>SADVAGAVIDGAGLGFDVLKTVLEALGNVKRKIAVGIDNESGRTWTAMNTYFRSGTSDIVLPHKVAHGKALLYNGQKNRGPVATGVVGVIAYSMSDGNTLAVLFSVPYDYNWYSNWWNVRVYKGQKRANQRMYEELYYHRSPFRGDNGWHSRSLGYGLKSRGFMNSSGHAILEIHVTKA[2x]

The multigene family of actinoporins are a group of cnidarian pore-forming toxins produced by sea anemones well known for their widespread polymorphism. Strongly influenced by negative selection, actinoporins have conserved important functional sites to ensure the preservation of their mechanism of pore formation, a complex process involving many different steps. The steps leading to pore formation comprise (1) the binding of the toxins to the cell membrane, (2) toxin diffusion across the membrane plane, (3) protein oligomerization, and (4) translocation of the N-terminal α-helices through the lipid bilayer.

The structure is composed of a β-sandwich core flanked by an N-terminal and a C-terminal α-helix. Relevant functional areas such as the lipid-binding region (contoured by a hydrophobic loop and the C-terminal α-helix) and the pore-forming N-terminal α-helix were conserved. When considering only the differences among fragaceatoxins, it is observed that FraE shared a high identity (98%) with FraC, explaining their similar activity above. The most stable isoforms were FraA and FraB as judged by their higher TM values (TMFraA = 65 ± 1 °C, TMFraB = 62 ± 2 °C), followed by FraC, FraD, and FraE (TMFraC = 53 ± 3 °C, TMFraD = 47 ± 1 °C, and TMFraE = 51 ± 1 °C). Differences in the exponential dependencies of the lag time on the protein concentration distinguish the more cooperative FraC and FraE from the other fragaceatoxin isoforms. In particular, these two proteins are predicted to have regions of larger, local intrinsic disorder, suggesting an underlying local flexibility that may enhance binding cooperativity. The overall hemolytic activities, however, are lower, implying that protein flexibility may obstruct other steps during the pore-forming process. Moreover, FraC and FraE share an identical N-terminal helix, although the hemolysis produced by the latter is considerably faster. Given the high sequence similarity between FraC and FraE, other possibilities such as long-range interactions may help to explain kinetic differences, such as those described for Stn-II. Similar mechanisms may apply to the arginine/aspartate difference at position 129 of FraC versus FraE.> PISPIETVPVKLKPGMDGPKVKQWPLTEEKIKALVEICTEMEKEGKISKIGPENPYNTPVFAIKKKDSTKWRKLVDFRELNKRTQDFWEVQLGIPHPAGLKKKKSVTVLDVGDAYFSVP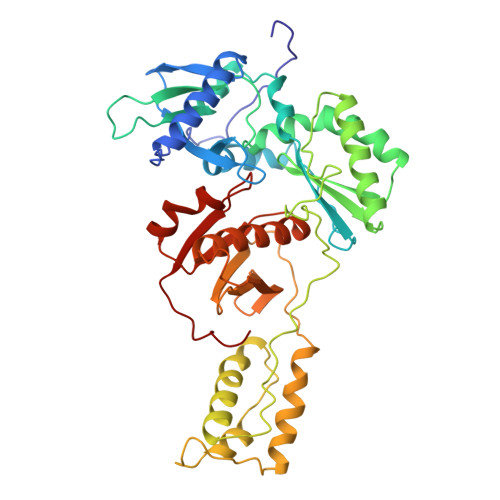LDEDFRKYTAFTIPSINNETPGIRYQYNVLPQGWKGSPAIFQSSMTKILEPFKKQNPDIVICQYMDDLYVGSDLEIGQHRTKIEELRQHLLRWGLTTPDKKHQKEPPFLWMGYELHPDKWTVQPIVLPEKDSWTVNDIQKLVGKLNWASQIYPGIKVRQLSKLLRGTKALTEVIPLTEEAELELAENREILKEPVHGVYYDPSKDLIAEIQKQGQGQWTYQIYQEPFKNLKTGKYARMRGAHTNDVKQLTEAVQKITTESIVIWGKTPKFKLPIQKETWETWWTEYWQATWIPEWEFVNTPPLVKLWY>[2x]MKEITLTIDGKVCKGVQGDTILDVANKNDVYIPTLCYQKGLTPIGACRMCVVQLEGNPKMLPSCTTPAQDGMVVVTKNEKLKDYRRQILELLFAGRNHFCMYCSQSGDCELQRLAIEHEMDSVRFPYLYEDFEVDATDPNLMMDHNRCVLCQRCIRTCSEIVGAHTLDLERRGWQAKVIADLGKRLRESDTCVNCGACAQSCPTGTITIREFAYRGRRSECDAVVESVCPLCAVGCKIKTYVRTGSIVRVEGTGVEEPDGGQLCHMGRWWLPESTERERVTVPLIREGASYREATWEEALALASAEFKKAYDQEKAGAILSSLCTDEELTLFSALFRNALKMKHIDTFDGDIIRGFFKGFMPFREQGVRPFTAAHHILDSDLIITMFADPQKEAPVVASYIRVACLHRNAKLMNLSYGPSPFPGLVDLDIRLPEGQAVPKALSNLAEIIGKISLGPSDMASFGEFEAGAGKALSSYRESIEESARAMGLDPKIAEEVALMLISARRPIFIIGGRATKSHELVTAACNLAVASKAFFEDGLGVVPLLVSANSLGARNTVVSENPWLGRERRDFLYVFSTAMVPEEEEILAAISATRFVVVQTPFKVRPLVNLADILLPAPAWYERSGHFCTIEGERRKLNTIVPPKGEIKSLHYVMDEFAKKLGVKLERPEVSPCEEIFKSQLRASEARIVTL;>MAIYRAHVLVCRGTGCTASGAPGVMKAFKEELAKKGLDREVMLVETGCHGMCEMGPVVVVYPEGAFYCRVTPEDVPEIVEEHLYKGRIVQRLLYTVPEDMEKVPYYKDIPFYSKQHRIVLSNCGYIDPEKIEEYIARDGYMALGKALLEMTPEEVLEEVKKSGLRGRGGAGFPTGLKWEFAKKASGDKKYVICNADEGDPGAFMDRSTLEGDPHSVIEGMTIGAYVIGADEGYIYCRAEYPLAIKRLKIAIAQAEEMGLLGDHIMGTNFSFHLHLKEGAGAFVCGEETALMASIEGRRGMPRPRPPFPAQHGLWGKPTNINNVETWANVPRIILNGADWFASMGTEKSKGTKIFALTGKITNTGLIEVPMGITIREIIYELGGGILNGKEFKAVQIGGPSGGCLTKEHLDLPIDYESLTAAGAIMGSGGLVVMDEDTCMVDVAKFFLEFTQRESCGKCVPCREGTKQMLLMLQKICNGEGTMDDLSKLEELAHMVKETSLCGLGQTAPNPVITTIRYFRDEYVAHIKDKRCPAKICPALIKYVVDPEKCRKCGLCARNCPVKCISGDRQTPYLINQEKCIKCGTCMQVCPFGAIGKV[2x];>MALSTVDVVEKVKEIVAPWKGKQGGLIPILQEVQRELGYLPEEALLTISRELKMPKAEVYGVATFYAQFHLKPRGRHVIRVCRGTACHVRGSLQILEKVKQMLGIEENETTDDLRFTLEPVACLGACGLAPVMMVDEDTHGRMTPDKIQAILDKYQ[2x];>[2x]MTEVFKLEINPVTRIEGHGKITVMLDESGHVRETRFHVTQYRGFEVFTHGRDFREMPVITPRICGICPVSHHLASAKACDEILGVTITPAAHKLRELMHMGQIVQSHALSFFHLSSPDILWGFDAPVKIRNVAGLVDRYPELAKKGIMLRKFGQEIIKTLGGKKIHPWHSIPGGVNRSLTPQERDAIAAQLPEMKSIAMEAIKLIKDYLQEGGEELKEFATLDTAYMGLVRDGYLELYDGEVRIKAPRGRILDQFDPKDYLDHIGEHVEPWSYLKFPFYKALGFPHGSYRVGPLARLNAADAVSTPEASKEFALYKEMGEDGIVPYTLYYHYARLIEALYGLERIEQLLADPDITSSDLRVTSKEINPEGIGVIEAPRGTLIHHYQVNESGVITKVNLIVATGHNNFAMNKGVEMVAKKYITGTNVPEGVFNRLEHVIRAYDPCLSCSTHAVGKMPLKLELVGPTGEILKEVTRD;>[2x]MAKAKVATFWLEACAGCHMSFLDLDERLIDLFQNVEILFSPIVDAKDIPNIDVGVLSGGLGNVEEVELAKKMRERCKYLVAWGDCAVFGGINCMRNFIPKDVVLREGYIETASTVNPQGIVPSEDIPELLPRALPIDYEVKVDVYVPGCPPDADTIYYVFKELLAGRVPKVPSEMMRYD

In summary, we have described the cryo-EM structure of NiFe-HydABCSL, an electron-bifurcating hydrogenase consisting of a conventional NiFe-hydrogenase module (SL subunits) and of a bifurcating module (ABC subunits) that is highly similar to a previously characterized bifurcating heterotrimeric FeFe-hydrogenase. We report cryo-EM structures of the related NiFe-HydABCSL hydrogenase that reversibly oxidizes H2 and couples endergonic reduction of ferredoxin with exergonic reduction of NAD. Here, we report cryo–electron microscopy (cryo-EM) structures of NiFe-HydABCSL determined in a flavin-free apo state, in an “electron bifurcation-ready” (BR) state, and in a “post-electron bifurcation” (PB) state. The structures of the NiFe-enzyme show that none of the previous proposals for the site of bifurcation in [FeFe]-HydABC hydrogenases are likely to be correct and that instead electron bifurcation occurs at a single NAD(H)-binding flavin in combination with a unique arrangement of three iron-sulfur clusters.

No density for the expected FMN was observed in the EM map, indicating that the as-purified complex is in the flavin-free apo state. Flavoenzymes typically have a lower affinity for flavin in their reduced states, and in this regard, the absence of FMN in the NiFe-HydB structure is consistent with the reduced state of HydSL in our structure. Therefore, NiFe-HydSL is in the reduced active state and brief air exposure during EM grid preparation did not oxidize the catalytic center. The NTD and CTD of NiFe-HydB were partially flexible, although EM densities were clearly visible. In the FMN-free apo state structure of NiFe-HydABCSL, the distances between the C1 and B2 [2Fe-2S] clusters (19 Å) and between B2 and the B3 [4Fe-4S] clusters (18 Å) are too far to transfer electrons. Substantial conformational changes must therefore occur when FMN and/or NAD bind to enable electron transfer from FMN to B3, and this is discussed below. However, B5 is close enough to the C1 cluster (11 Å) for electron transfer in the FMN-free apo state, so the possibility of B5 being involved in electron transfer to Fd cannot be entirely ruled out. Direct electron transfer between B1 and C1 is highly unlikely based on our structure, as the closest (side-to-side) distance between them is more than 22 Å, which is too far for electron transfer to occur. The HydC CTD position is stabilized by the HydB NTD in the FMN-free apo state, and the movement of the HydC CTD during the bifurcation process needs the HydB NTD to be released. In the absence of NAD and FMN, the HydB CTD is disordered, while the HydC CTD is stable.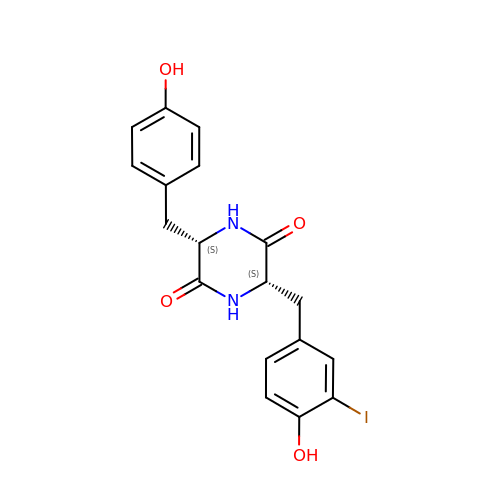(3~{S},6~{S})-3-[(4-hydroxyphenyl)methyl]-6-[(3-iodanyl-4-oxidanyl-phenyl)methyl]piperazine-2,5-dione | C18 H17 I N2 O4 | NQIPTQNZLHTHOS-GJZGRUSLSA-N> GHRTLASTPALWASIPCPRSELRLDLVLPSGQSFRWREQSPAHWSGVLADQVWTLTQTEEQLHCTVYRGDKSQASRPTPDELEAVRKYFQLDVTLAQLYHHWGSVDSHFQEVAQKFQGVRLLRQDPIECLFSFICSSNNNIARITGMVERLCQAFGPRLIQLDDVTYHGFPSLQALAGPEVEAHLRKLGLGYRARYVSASARAILEEQGGLAWL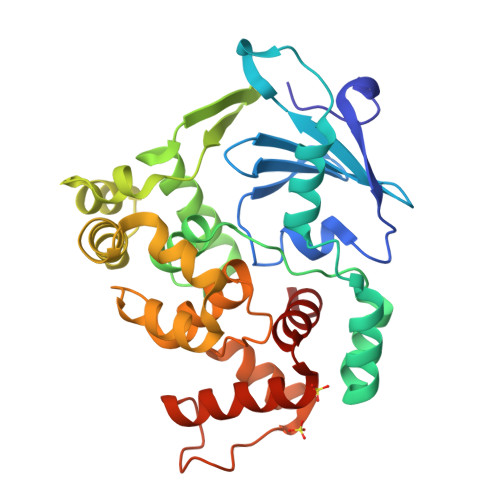QQLRESSYEEAHKALCILPGVGTKVADCICLMALDKPQAVPVDVHMWHIAQRDYSWHPTTSQAKGPSPQTNKELGNFFRSLWGPYAGWAQAVLFSADL>TMGSGRIFQIPEETIKCQPFECPDHFYVIDAQDFGWNHPQAHIQLWWDKDADVFYLARVWKKSENTAVQAWGAVKSWANKIPVAWPHDGHQHEKGGGEQLKTQYADAGFSMLPDHATFPDGGNSVESGISELRDLMLEGRFKVFNTCEPFFEEFRLYHRDENGKIVKTNDDVLDATRYGYMMRRFARMMRDIRKPKEKKIPAPIRPVRRGR[4x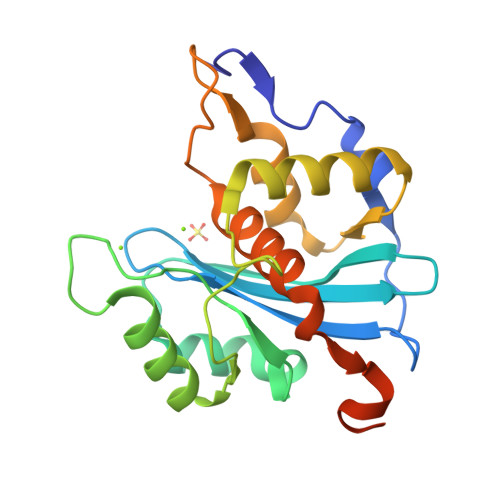]>[3x]MNLTDSLQNVLSGVGTLNRYRLDIPSCPSSLDVEDFSGTEGISKIYRYDIIFTSTDRYPDAAWFLRKSATLIMGTGLLESLTEQKKVHGVITDFRRISGSEDQAQYRITLKPFISLLDKQFRTHRFFVNKSVPEVVEQILTEHGLKGWEYEFSLKRTYPKREQINQYQESDLRFIQRLLAEVGIFYFFTLHPDAQTEVIHFGDVQAALIFDKTLPVNSPSGMSDSGTDSVWALNVEHRVVESRVITNDYNHREAQNILMSVPADMTRGEGYDTSYGEVYHYRPRHTERGDKIDPAPETANFWARLDHERFLAEQTRITGKSTDASLL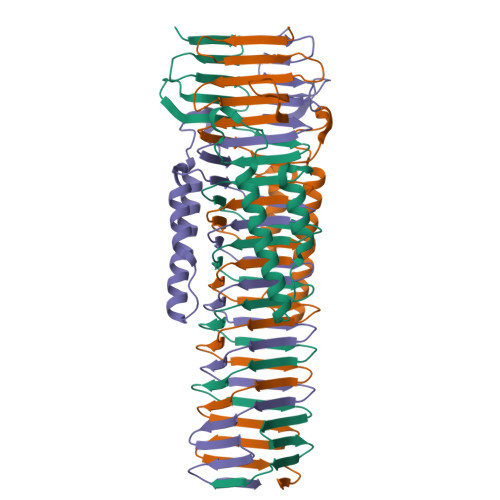PAQVLTITDSTPPVLPAPLQEPVLLTQLLFTGSRKSALQVMLSAVPYSEIVCWRPPLLTRPKITGTMTARVTSAKEGDIYAWQDASGMYRVKFDADRDDKNPGQESMPVRLAKPYSGDAYGFHFPLIQGTEVAIAFEEGDPDRPYIAHALHDSRHVDHVTDKNGTRNVIRTPANNKLRMEDKRGEEHIKLSTEYGGKTQLNLGHNVDASRELRGEGAELRTDDWISIRGGKGIFISADMQPQAQGKMLDMDEAIRQLEQALSLARSMAKAATAANATQGDISCQQRLNASLTDLTAPGMLLHAPDGIGMVSARALRIASGSESVGIMSGDNTDITAGQSFTVVAEGAVSLLSRNQGMQLLAAKGRVNIQAQSDDLSMSSQQNLDIQSSEGKVTVSANQELILACGGAYIKLSGGNIELGCPGQILLKSTNMQKMGPTSLDIASVEMPRGFGGGFILTDEAGVPQPSTPYRLTTAEGDILQGITDENGKTAPVNTSIPSVVKVEFGKVKIHGETE> GSMADEATRRVVSEIPVLKTNAGPRDRELWVQRLKEEYQSLIRYVENNKNAD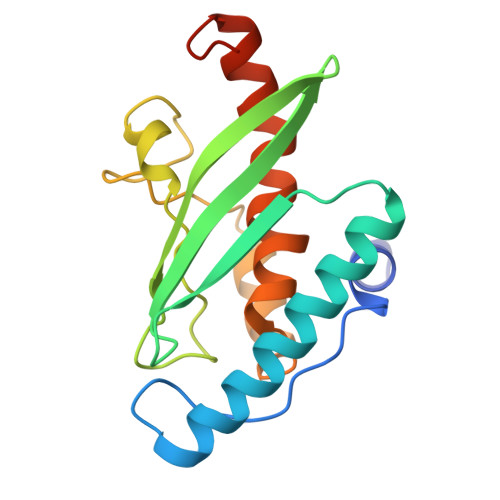NDWFRLESNKEGTRWFGKCWYIHDLLKYEFDIEFDIPITYPTTAPEIAVPELDGKVAKMYRGGKICLTDHFKPLWARNVPKFGLAHLMALGLGPWLAVEIPDLIQKGVIHHKEKCNQ>[2x]MGSSHHHHHHSSGLVPRGSMNEAEHSVEHPPVQGSHVEGGVVEHPDAKDFGSAAALPADPTWFKHAVFYEVLVRAFFDASADGSGDLRGLIDRLDYLQWLGIDCIWLPPFYDSPLRDGGYDIRDFYKVLPEFGTVDDFVALVDAAHRRGIRIITDLVMNHTSESHPWFQESRRDPDGPYGDYYVWSDTSERYTDARIIFVDTEESNWSFDPVRRQFYW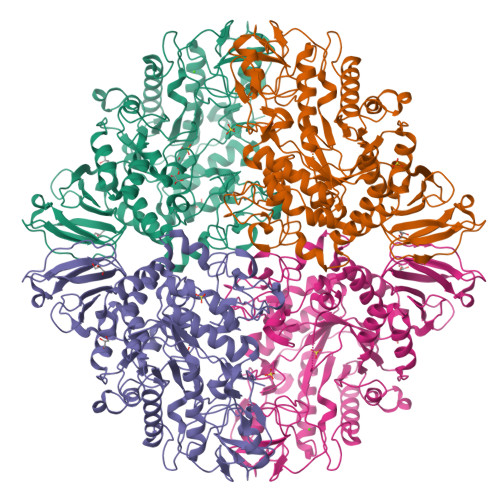HRFFSHQPDLNYDNPAVQEAMIDVIRFWLGLGIDGFRLDAVPYLFEREGTNCENLPETHAFLKRVRKVVDDEFPGRVLLAEANQWPGDVVEYFGDPNTGGDECHMAFHFPLMPRIFMAVRRESRFPISEIIAQTPPIPDMAQWGIFLRNHDELTLEMVTDEERDYMYAEYAKDPRMKANVGIRRRLAPLLDNDRNQIELFTALLLSLPGSPVLYYGDEIGMGDVIWLGDRDGVRIPMQWTPDRNAGFSTANPGRLYLPPSQDPVYGYQAVNVEAQRDTSTSLLNFTRTMLAVRRRHPAFAVGAFQELGGSNPSVLAYVRQVAGDDGDTVLCVNNLSRFPQPIELDLQQWTNYTPVELTGHVEFPRIGQVPYLLTLPGHGFYWFQLTTHEVGAPPTCGGERRL> GAMDPMRQSSLKKDWFLSEEEFKLWNRLYRLRDSDEIKEITLPQVQFSSLQNEENKPAQESTTGIHQLSLSEWRLWQDHPLPTHQVDHSDRCRHFIGLMQMIEGMRHEEGECSYELEVESYLQMEDVTSTFIAPR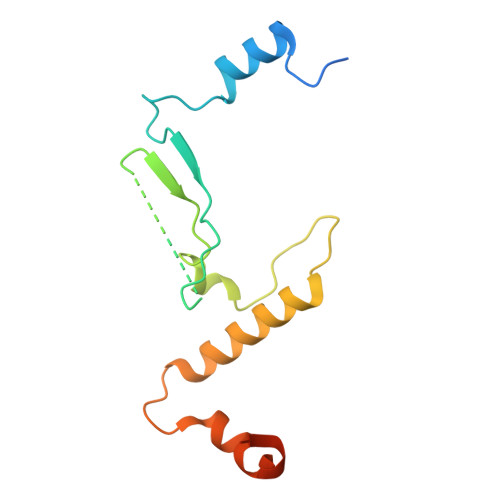NE>GAMDPSSPNYDKWEMERTDITMKHKLGGGQYGEVYEGVWKKYSLTVAVKTLKEDTMEVEEFLKEAAVMKEIKHPNLVQLLGVCTREPPFYIITEFMTYGNLLDYLRECNRQEVSAVVLLYMATQISSAMEYLEKKNFIHRDLAARNCLVGENHLVKVADFGLSRLMTGDTYTAHAGAKFPIKWTAPESLAYNKFSIKSDVWAFGVLLWEIATYGMSP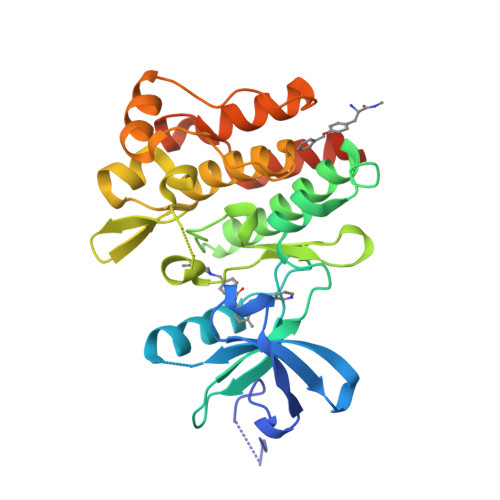YPGIDLSQVYELLEKDYRMERPEGCPEKVYELMRACWQWNPSDRPSFAEIHQAFETMFQESSISDEVEKELGKRGT[4x]> HHHHHHEVLLRSTETGQLLR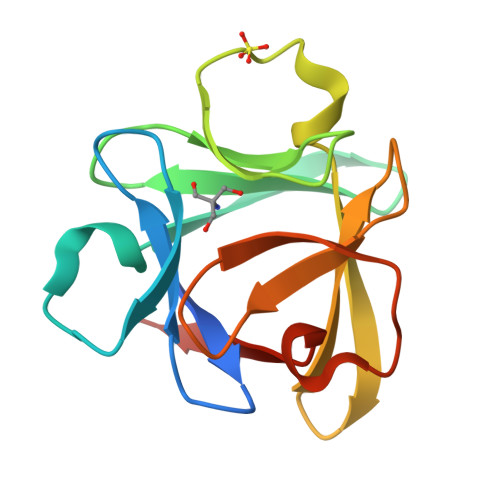INPDGTVDGTRDRSDPGIQLQISPEGNGEVLLRSTETGQLLRINPDGTVDGTRDRSDPGIQLQISPEGNGEVLLRSTETGQLLRINPDGTVDGTRDRSDPGIQLQISPEGNG> KPSASNLIWSDEPAVVVYPQEDKNSEGSFGKYRKPASVWEAEGYPIGNGRVGAMIFSAPGRERLALNEISLWSGGANPGGGYGYGPDAGTNQFGNYLPFGDLFVDFKKGDQPASLSVEDFTRSLDLRDGIHKVNYKADGVTYDREAFSSTPANVLVLNYKASKPGQFSADFSVNSQLGADISAKGSVITWKGMLKNGMNYEGRVLIRPKGGTLSASGDKISVKNADSCMVVIAMETDYLMDYKKDWKGESPSRKLDRYAAKAASADYAALKQAHISQYKSMFDRVKVNFGKTEEDVAKLPTPKRLEAYKKNPADPDLEETMFQFGRYLLLSSSRPGTLPANLQGLWNDYVKPPWACDYHNNINVQMAYWGAEPANLSECHEALVNYVEAMAPGCRDASQANKGFNTKDGKPVRGWTVRTSQNIFGGNGWQWNIPGAAWYALHIWEHYAFTGDRKYLEKQAYPLMKEICHFWEDHLKELGAGGEGFKTNGKDPSEEEKK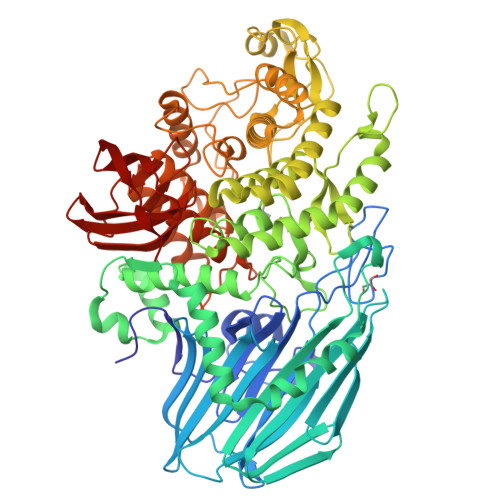DLADVKAGTLVAPNGWSPEHGPREDGVMHDQQLIAELFSNTIKAARILGKDAAWAKSLEGKLKRLAGNKIGKEGNLQEWMIDRIPKTDHRHTSHLFAVFPGNQISKLKTPKLAEAARLSLEWRGTTGDSRRSWTWPWRTALWARLGEGNKAHEMVQGLLKFNTLPNMLTTHPPMQMDGNFGIVGGICEMLVQSHAGGLDIMPSPVEAWPEGSVKGLKARGNVTVDFSWKDGKVSNVKLYSAQPKVLPVRVNGKMTRMKTLPLK> MKLLLFGYGNVGKAFRKLLHEKRSPELNDVIIGGIVTRRGIMLQDKEDFTPDLEGDVFKAFEKIKPDIIVDVSSANYNNGEPSLSLYKEAIKDGVNIITTNKAPLALAFNEIFSLARSKGVKIGFQGTVMSGTPSINLYRVLPGSRVIKIRGILNGTTNFILTLMNKGVSFEEALKEAQRRGYAEEDPTLDINGFDAAAKITILANFMIGNSVTIKDVKFEGINRDLPKNEKIKLIAYADEKEVWVKPLPISQDDPLYNVDGVENALEITTDIQSILIRGPGAGPVNAAYGALSDLILLKRDCL

Within the aspartate pathway to threonine, methionine and isoleucine synthesis, homoserine dehydrogenase (HSD) functions in the third reaction step – i.e., NAD(P)H-dependent production of homoserine from L-aspartate-4-semialdehyde. We previously reported that the HSD from the hyperthermophilic archaeon Sulfolobus tokodaii (StHSD) is activated by reductive cleavage of the disulfide bond formed between cysteine residues (Cys304) in the C-terminal regions of the homodimer subunits. The crystal structure revealed that StHSD is composed of a nucleotide-binding region (residues 1–130 and 285–304), a dimerization region (residues 131–145 and 256–284), and a catalytic region (residues 146–255). In the present study, we discovered the marked inhibition of StHSD by cysteine and present structural evidence that a cysteine binds at the active site of StHSD in complex with NAD.

To determine the structural features of cysteine’s inhibition of StHSD, we examined the crystal structure of StHSD in complex with cysteine and NAD at 2.1 Å resolution. The overall structure clearly showed the presence of a disulfide bond formed between two cysteine residues (position 304) in the C-terminal regions of the two subunits, suggesting that the structure is the less active oxidized form. Superposition of the native and ligand bound structures showed that a large conformational change occurs upon ligand binding, which affects the catalytic region (amino acids 146–255) in particular. Ligand binding induced much less displacement of the nucleotide binding region than the catalytic region (amino acids 146–255). Surprisingly the structural analysis showed that cysteine locates within the homoserine binding site within the StHSD-NAD complex, where it interacts with six amino acid residues (Lys102, Gly156, Thr157, Tyr183, Glu185 and Asp191). Interestingly, the distance between the sulfur atom of cysteine and the C4 atom of the nicotinamide ring of NAD was calculated to be 1.9 Å, which is sufficiently close to form a covalent bond. We suggest this binding increases the binding affinity of cysteine for the active site. Considering that the significant conformational change of the loop is induced by the cysteine binding, the displacement of the loop may have important role for cysteine binding. The bulky and hydrophobic side chain of Phe49 could exclude the C2′ phosphate group of NADP so that Phe49 may be responsible for the low activity toward NADP.>MGSSHHHHHHGSPVRASIEPLTWENAFFGVNSAIVRITSEAPLLTPDALAPWSRVQAKIAASNTGELDALQQLGFSLVEGEVDLALPVNNVSDSGAVVAQETDIPALRQLASAAFAQSRFRAPWYAPDASGRFYAQWIENAVRGTFDHQCLILRAASGDIRGYVSLRELNATDARIGLLAGRGAGAELMQTALNWAYARGKTTLRVATQMGNTAAL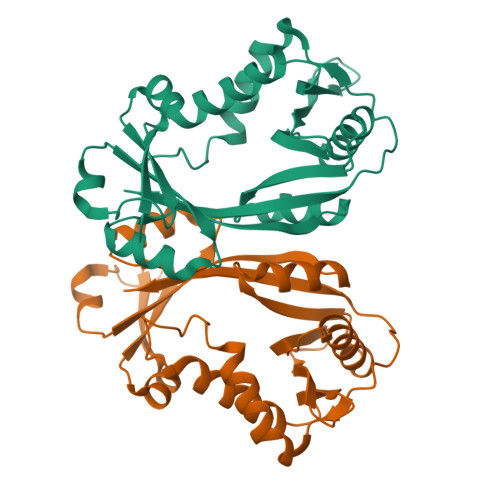KRYIQSGANVESTAYWLYR[2x]> MKVNPNNIELIISAVKEEQYPETELSEVALSGRSNVGKSTFINSMIGRKNMARTSQQPGKTQTLNF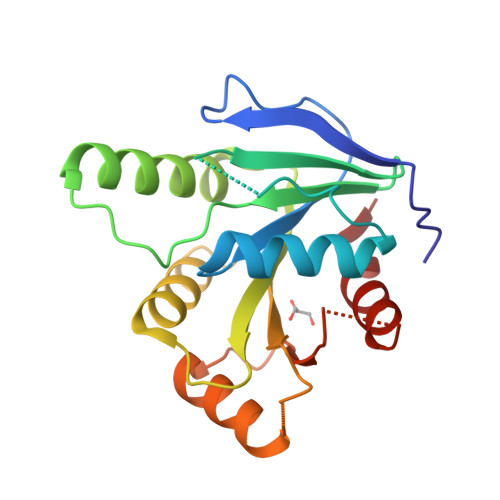YNIDEQLIFVDVPGYGYAKVSKTQREKFGKMIEEYITKRENLQLVIQLVDLRHDPTQDDILMYNYLKHFDIPTLVICTKEDKIPKGKVQKHIKNIKTQLDMDPDDTIVSYSSIQNNKQQQIWNLIEPYIS>[2x]PPKLCLVCSDEASGCHYGVLTCGSCKVFFKRAVEGQHNYLCAGRNDCIIDKIRRKNCPACRYRKCLQAGMNLEA

The GR is a ligand-regulated transcription factor (TF) that controls the expression of thousands of genes. GR has a domain structure common to the NR superfamily: an unstructured N-terminal domain, a zinc finger (ZnF)-containing DNA-binding domain (DBD), a hinge region and a ligand-binding domain. To modulate transcription, GR binds directly to DNA at canonical GBSs composed of two pseudo-palindromic hexameric repeats separated by a 3-bp spacer (5′-AGAACAnnnTGTTCT-3′). GR binds a canonical GBS as a dimer oriented in a head-to-head fashion.

Next, we biochemically characterize the extant human GR (hereafter GR, unless labeled otherwise) DBD bound to an unmethylated CpG-containing GBS (pre-GBS) and its methylated counterpart (5mC-GBS) and find that GR has preference for the 5mCpG GBS over the pre-GBS. Binding to the 5mC-GBS and pre-GBS showed Kd values of 131 and 206 nM, respectively. To determine how GR recognizes the 5mC-GBS and pre-GBS, we solved crystal structures of the GR DBD–5mC-GBS and GR DBD–pre-GBS complexes at a resolution of 2.0 and 2.5 Å, respectively. Both complexes crystallized in the C 1 2 1 space group and each structure contains a dimer of DBD protein molecules in the asymmetric unit. We found that in the 5mC-GBS structure, Arg447 makes side-on hydrophobic contacts with the methyl group of the 5mC, mimicking interactions with a thymine base seen in extant GBSs. This hydrophobic interaction is lost in the GR DBD–pre-GBS complex that contains an unmodified cytosine base at this position. Without this interaction, Arg447 in monomer B moves outward but still makes hydrogen bonds with the guanine in CpG dinucleotide by one amide group, suggesting the methyl-derived side-on contact helps stabilize the Arg447. Each GR DBD monomer contacts the methylated pre-GBS with one more van der Waals contact than with an unmethylated pre-GBS, which results in larger buried solvent accessible surface area (BASA) between GR DBD and nucleotides in each half-palindromic site (140 Å2 versus 109 Å2 and 125 Å2 versus 115 Å2). The affinity between GR and pre-GBS (206 nM) suggests the pre-GBS may be a functional glucocorticoid response element (GRE) as it is a variation of TpG-containing GBS.> MTVTRRHFLKLSAGAAVAGAFTGLGLSLAPTVARAELQKLQWAKQTTSICCYCAVGCGLIVHTAKDGQGRAVNVEGDPDHPI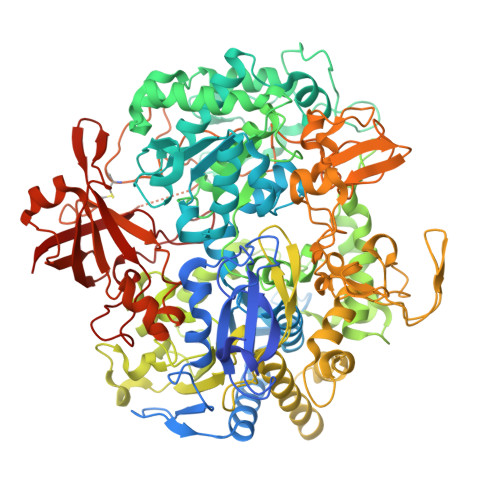NEGSLCPKGASIFQLGENDQRGTQPLYRAPFSDTWKPVTWDFALTEIAKRIKKTRDASFTEKNAAGDLVNRTEAIASFGSAAMDNEECWAYGNILRSLGLVYIEHQARIUHSPTVPALAESFGRGAMTNHWNDLANSDCILIMGSNAAENHPIAFKWVLRAKDKGATLIHVDPRFTRTSARCDVYAPIRSGADIPFLGGLIKYILDNKLYFTDYVREYTNASLIVGEKFSFKDGLFSGYDAANKKYDKSMWAFELDANGVPKRDPALKHPRCVINLLKKHYERYNLDKVAAITGTSKEQLQQVYKAYAATGKPDKAGTIMYAMGWTQHSVGVQNIRAMAMIQLLLGNIGVAGGGVNALRGESNVQGSTDQGLLAHIWPGYNPVPNSKAATLELYNAATPQSKDPMSVNWWQNRPKYVASYLKALYPDEEPAAAYDYLPRIDAGRKLTDYFWLNIFEKMDKGEFKGLFAWGMNPACGGANANKNRKAMGKLEWLVNVNLFENETSSFWKGPGMNPAEIGTEVFFLPCCVSIEKEGSVANSGRWMQWRYRGPKPYAETKPDGDIMLDMFKKVRELYAKEGGAYPAPIAKLNIADWEEHNEFSPTKVAKLMNGYFLKDTEVGGKQFKKGQQVPSFAFLTADGSTCSGNWLHAGSFTDAGNLMARRDKTQTPEQARIGLFPNWSFCWPVNRRILYNRASVDKTGKPWNPAKAVIEWKDGKWVGDVVDGGGDPGTKHPFIMQTHGFGALYGPGREEGPFPEHYEPLECPVSKNPFSKQLHNPVAFQIEGEKKAVCDPRYPFIGTTYRVTEHWQTGLMTRRCAWLVEAEPQIFCEISKELAKLRGIGNGDTVKVSSLRGALEAVAIVTERIRPFKIEGVDVHMVGLPWHYGWMVPKNGGDTANLLTPSAGDPNTGIPETKAFMVDVRKV In Gram-positive pathogens such as Staphylococcus aureus (Sa) and Enterococcus faecalis (Ef), the pleiotropic transcription factor CodY plays a key role in integrating metabolism and virulence factor expression. CodY DNA-binding is activated by two types of ligands: branched chain amino acids (BCAAs, i.e. isoleucine, leucine, and valine) and, in most cases, guanosine triphosphate, GTP. Each 30 kDa protomer comprises the N-terminal ligand-binding domain called GAF (cGMP-specific phosphodiesterases, adenylyl cyclases and FhlA). The GAF domain is connected by an extended linker helix to the C-terminal DNA-binding (DBD) domain that contains a winged helix-turn-helix (wHTH) motif.

Unexpectedly however, the structures revealed a previously undescribed monomeric form of SaCodY and a dimeric EfCodY. The GAF domains of the ligand-free EfCodY protomers pack with close to perfect 2-fold symmetry. However, this symmetry breaks down in the C-terminal part of the linker helices as well as the DBD domains, which all assume different orientations in the four protomers in the asymmetric unit. Furthermore, for protomer chain C, parts of the linker helix and the DBD domain could not be modelled (residues 181–260). This evidenced the flexibility of them in the ligand-free EfCodY, in consistency with previous structures of CodY. In ligand-free EfCodY, residues Leu60-Gln78/Glu55-Ser73 (EfCodY/SaCodY sequence numbering = shift –5) form an extended loop with a few loop residues involved in crystal contacts. The fold of the loop in all four protomers is identical even though the crystal contacts are not identical, suggesting that the loop structure in the crystal structure also represents the structure in solution. The most apparent difference of the loop structure to that in SaCodY is the absence of helix H3. Nevertheless, Lys74 (Arg69 in SaCodY) extends into the vacant Leu binding pocket.

>GAMATLLEKTRQVNELLQKNNLFDVQAELPYNKMAMILGDILESNAYIISSSGDLLGYTEKLDVNNARIKNMFKEKKFPQGYTEAVDMLKVTEANIPIDSDLTAFPFESRELYPFGLTTIVPLYGAGKRLGTIILARVEKSFNEDDLVLAEYSATVVGMQILYHQSRTIEAEVRSATAVQMAINTLSYSELKAVHAIFEALDGEEGRLTASSIADEIGITRSVIVNALRKLESAGIIESRSLGMKGTYLKVLNQQFIKELEK[4x]(4R)-4-[3-(2-fluoropyridin-3-yl)phenyl]-4-(4-methoxyphenyl)-4,5-dihydro-1,3-oxazol-2-amine | 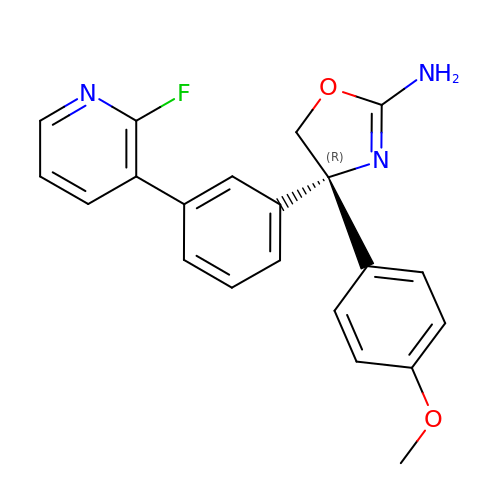C21 H18 F N3 O2 | WCJQDRXUNINKDD-OAQYLSRUSA-N>[4x]MSQHNEKNPHQHQSPLHDSSEAKPGMDSLAPEDGSHRPAAEPTPPGAQPTAPGSLKAPDTRNEKLNSLEDVRKGSENYALTTNQGVRIADDQNSLRAGSRGPTLLEDFILREKITHFDHERIPERIVHARGSAAHGYFQPYKSLSDITKADFL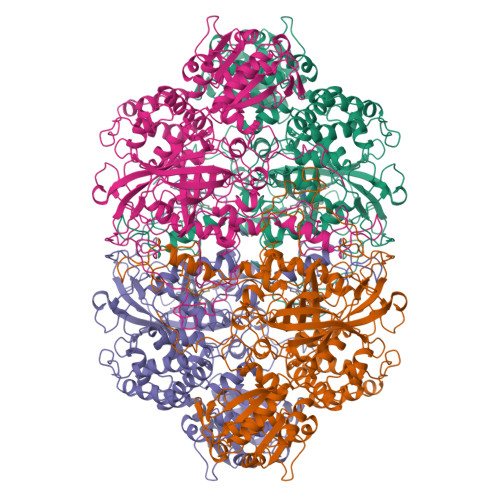SDPNKITPVFVRFSTVQGGAGSADTVRDIRGFATKFYTEEGIFDLVGNNTPIFFIQDAHKFPDFVHAVKPEPHWAIPQGQSAHDTFWDYVSLQPETLHNVMWAMSDRGIPRSYRTMEGFGIHTFRLINAEGKATFVRFHWKPLAGKASLVWDEAQKLTGRDPDFHRRELWEAIEAGDFPEYELGFQLIPEEDEFKFDFDLLDPTKLIPEELVPVQRVGKMVLNRNPDNFFAENEQAAFQPGHIVPGLDFTNDPLLQGRLFSYTDTQISRLGGPNFHEIPINRPTCPYHNFQRDGMHRMGIDTNPANYEPNSINDNWPRETPPGPKRGGFESYQERVEGNKVRERSPSFGEYYSHPRLFWLSQTPFEQRHIVDGFSFELSKVVRPYIRERVVDQLAHIDLTLAQAVAKNLGIELTDDQLNITPPPDVNGLKKDPSLSLYAIPDGDVKGRVVAILLNDEVRSADLLAILKALKAKGVHAKLLYSRMGEVTADDGTVLPIAATFAGAPSLTVDAVIVPCGNIADIADNGDANYYLMEAYKHLKPIALAGDARKFKATIKIADQGEEGIVEADSADGSFMDELLTLMAAHRVWSRIPKIDKIPA> MGKYLLPTAAAGLLLLAAQPAMDFTIQDIRVEGLQRTEPSTVFNYLPVKVGDTYNDTHGSAIIKSLYATGFFDDVRVETADGQLLLTVIERPTIGSLNITGAKMLQNDAIKKNLESFGLAQSQYFNQATLNQA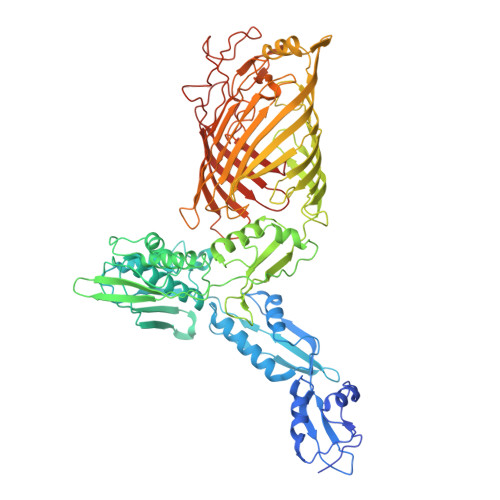VAGLKEEYLGRGKLNIQITPKVTKLARNRVDIDITIDEGKSAKITDIEFEGNQVYSDRKLMRQMSLTEGGIWTWLTRSDRFDRQKFAQDMEKVTDFYQNNGYFDFRILDTDIQTNEDKTRQTIKITVHEGGRFRWGKVSIEGDTNEVPKAELEKLLTMKPGKWYERQQMTAVLGEIQNRMGSAGYAYSEISVQPLPNAGTKTVDFVLHIEPGRKIYVNEIHITGNNKTRDEVVRRELRQMESAPYDTSKLQRSKERVELLGYFDNVQFDAVPLAGTPDKVDLNMSLTERSTGSLDLSAGWVQDTGLVMSAGVSQDNLFGTGKSAALRASRSKTTLNGSLSFTDPYFTADGVSLGYDIYGKAFDPRKASTSVKQYKTTTAGGGVRMGIPVTEYDRVNFGLAAEHLTVNTYNKAPKRYADFIRKYGKTDGADGSFKGLLYKGTVGWGRNKTDSASWPTRGYLTGVNAEIALPGSKLQYYSATHNQTWFFPLSKTFTLMLGGEVGIAGGYGRTKEIPFFENFYGGGLGSVRGYESGTLGPKVYDEYGEKISYGGNKKANVSAELLFPMPGAKDARTVRLSLFADAGSVWDGRTYTAAENGNNKSVYSENAHKSTFTNELRYSAGGAVTWLSPLGPMKFSYAYPLKKKPEDEIQRFQFQLGTTF>[4x]GMITSIARQSIILKCLRQKSVLVSNYELYYTAGLAKKCFGIAVDADMEP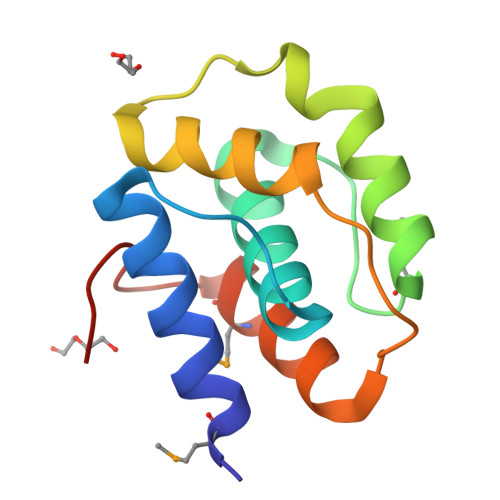KQLLEELQKHIDKVSPADEQEKYLIHLLGNYEPDDTHDEQTVELFHMGETEEHIWQVSIT> ATGGGGCGGGGCT;> TAGCC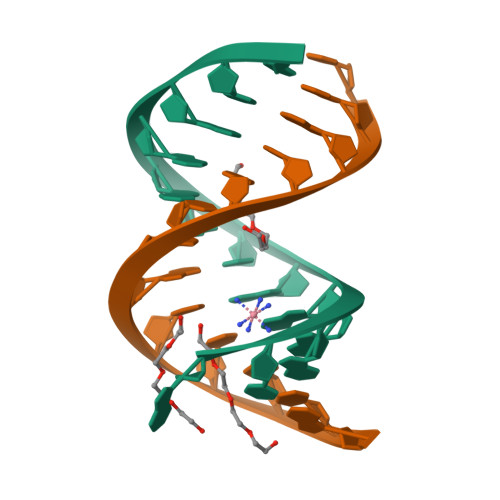CCGCCCCA>[2x]GGCCAGUAUAACCUCAAUGAU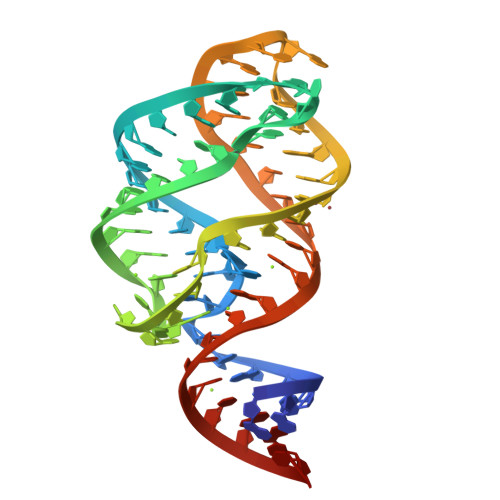AUGGUUUGAGGGUGUCUACCAGGAACCGUAAAAUCCUGACUACUGGUCX>[2x]MSKGTTSQDAPFGTLLGYAPGGVAIYSSDYSSLDPQEYEDDAVFRSYIDDEYMGHKWQCVEFARRFLFLNYGVVFTDVGMAWEIFSLRFLREVVNDNILPLQAFPNGSPRAPVAGALLIWDKGGEFKDTGHVAIITQLHGNKVRIAEQNVIHSPLPQGQQWTRELEMVVENGCYTLKDTFDDTTILGWMIQTEDTEYSLPQPEIAGELLKISGARLENKGQFDGKWLDEKDPLQNAYVQANGQVINQDPYHYYTITESAEQELIKATN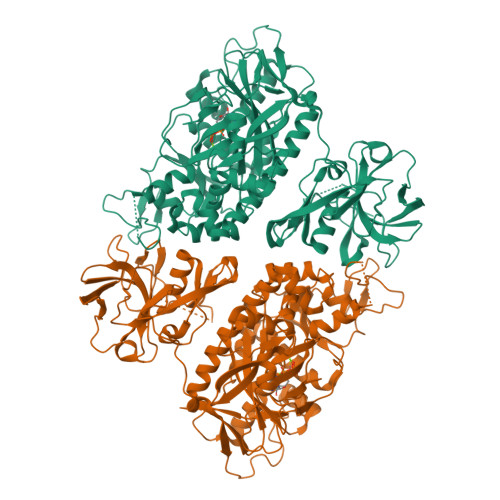ELHLMYLHATDKVLKDDNLLALFDIPKILWPRLRLSWQRRRHHMITGRMDFCMDERGLKVYEYNADSASCHTEAGLILERWAEQGYKGNGFNPAEGLINELAGAWKHSRARPFVHIMQDKDIEENYHAQFMEQALHQAGFETRILRGLDELGWDAAGQLIDGEGRLVNCVWKTWAWETAFDQIREVSDREFAAVPIRTGHPQNEVRLIDVLLRPEVLVFEPLWTVIPGNKAILPILWSLFPHHRYLLDTDFTVNDELVKTGYAVKPIAGRCGSNIDLVSHHEEVLDKTSGKFAEQKNIYQQLWCLPKVDGKYIQVCTFTVGGNYGGTCLRGDESLVIKKESDIEPLIVVKK> MSGQNNVVGVHYKVGRRIGEGSFGVIFEGTNLLNNQQVAIKFEPRRSDAPQLRDEYRTYKLLAGCTGIPNVYYFGQEGLHNVLVIDLLGPSLEDLLDLCGRKFSVKTVAMAAKQMLARVQSIHEKSLVYRDIKPDNFLIGRPNS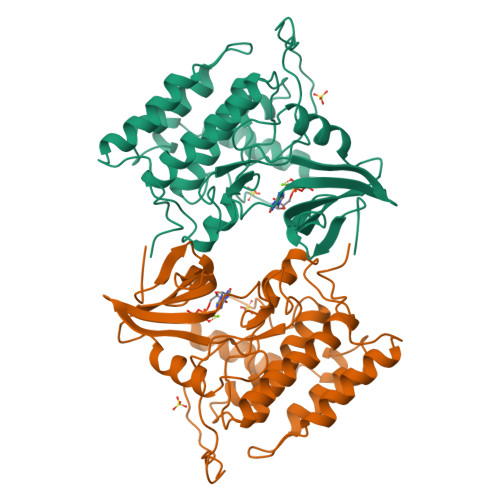KNANMIYVVDFGMVKFYRDPVTKQHIPYREKKNLSGTARYMSINTHLGREQSRRDDLEALGHVFMYFLRGSLPWQGLKAATNKQKYERIGEKKQSTPLRELCAGFPEEFYKYMHYARNLAFDATPDYDYLQGLFSKVLERLNTTEDENFDWNLL>MRTFTIRNNCPFTIWPAHFTNPDSPTKLTSQVAGWDAPARSQKSFQVPDRWAGRFWGRRNCDFSKQGPSSCATGGCNGGLICDARTGSGVPPATLAEFKLNGDGGKDYYDVSNVDGSNLPVLISNNKGCPSPSCRVDLNPGCPEDRMKVKDGRGTTIGCLSACQANLDGNHGNSANCCTGSHGKPETCPKTGVKYYDYFKGKCPDAYAYAYDESSQSALWTCNKGADYTVTFCPHHHH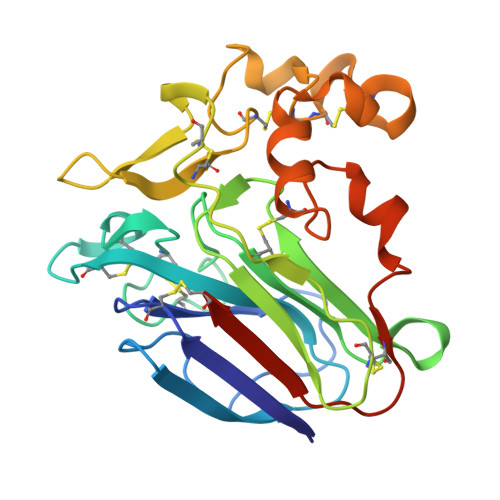HH[2x]>MERAIQGNDTREQANGERWDGGSGGITSPFKLPDESPSWTEWRLYNDETNSNQDNPLGFKESWGFGKVVFKRYLRYDRTEASL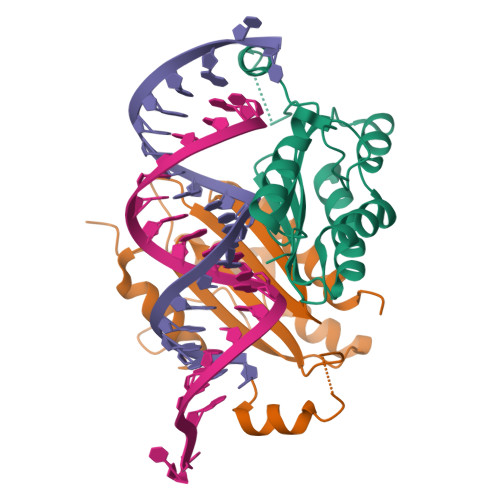HRVLGSWTGDSVNYAASRFLGANQVGCHYSIRFRGVSVTISGGSRTLQHLCEMAIRSKQELLQLTPVEVESNVSRGCPEGIETFKKESE[2x]5'-O-[(S)-hydroxy{[(R)-hydroxy({(S)-hydroxy[(1S)-1-(2-nitrophenyl)ethoxy]phosphoryl}oxy)phosphoryl]oxy}phosphoryl]adenosine | C18 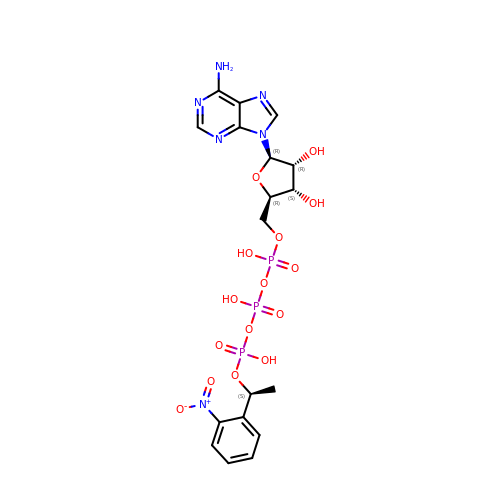H23 N6 O15 P3 | UOLVQBSMMHANLG-YBGGAFRISA-N>[2x]MGKIATKYHGDIEIHEKDIVRFEQ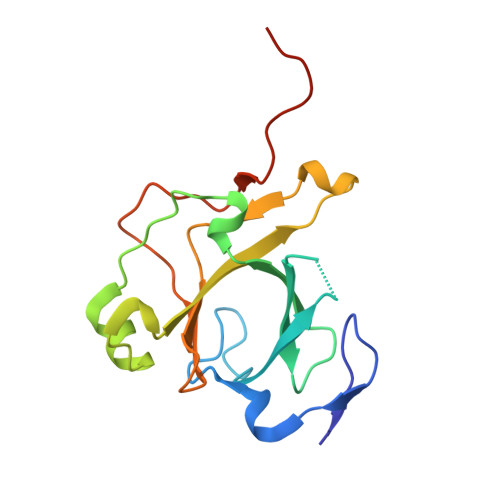GIPGFLEEKQFVLLQLEDTPFIILQSVNTPALGFVLIEPFSYFPTYEIDLDDNTLEQLQITGEQDVALYVILTVADPFDDTTANLQAPIVINVHKRLGKQVILTNTNYKTKHRLFPEKVAKHHHHHH Tyrosinases (EC.1.14.18.1) are bifunctional metalloenzymes catalyzing two sequential enzymatic reactions: hydroxylation of monophenols to o-diphenols (monophenolase activity) and oxidation of o-diphenols to the corresponding o-quinones (diphenolase or catecholase activity). The tyrosinase from the bacterium Verrucomicrobium spinosum (vsTyr) is produced as a pre-pro-enzyme in which a C-terminal extension serves as an inactivation domain. It does not require a caddie protein for copper ion incorporation, which makes it similar to eukaryotic tyrosinases. To gain an understanding of the catalytic machinery and regulation of vsTyr activity, we determined the structure of the catalytically active “core domain” of vsTyr by X-ray crystallography.

Crystals of the vsTyr core domain belong to the space group C2 containing two monomers per asymmetric unit. Despite reconstitution with CuSO4 after its purification, the initial crystal structure, determined by molecular replacement at 1.43 Å resolution, revealed that the copper sites were only partially occupied. Using the anomalous contribution of the Cu ions, occupancies of the CuA and CuB sites for the two copies of vsTyr per asymmetric unit could be estimated to be ~40% and ~80%, respectively. The lower occupancy observed for the A site may be caused by its proximity to His86, which belongs to a flexible loop. For vsTyr, the distances of 3.7 Å and 4.0 Å observed in the structures determined from unsoaked and CuSO4-presoaked crystals, respectively, fall within the 3.2–4.0 Å range that is characteristic for the met form. Interestingly, the increased metal site occupancy is the only noticeable difference between the two vsTyr core domain structures reported here. Their superposition results in a very low RMSD of 0.4 Å and identical crystal packing, hinting at the remarkable structural stability of the vsTyr core domain. The final models contain all amino acids of the crystallized construct, except for the C-terminal two (unsoaked) and three amino acids (soaked) in chains B, respectively.

>[2x]QSAKYHRLNLQNPAAAPFLESYKKAITVMLQLPPSDARNWYRNAFIHTLDCPHGNWWFVVWHRGYTGWFERTVRELSGDPNFAFPYWDWTALPQVPDSFFNGVLDPNNPAFIASYNEFYSQLSNPMSALWNSFSTAQLQQMRNRGFQSVNDVWQAVRDSPMFFPRGRARTLTRQNPGFDATTRRAVSIGTIRNALAPTDFITFGSGKTANHSESATQGILESQPHNNVHNNIGGFMQDLLSPTDPVFFAHHSNIDRLWDVWTRKQQRLGLPTLPTGANLPLWANEPFLFFIGPDGKPVAKNKAGDYATIGDFDYNYEPGSGEAV> GAMGSMNLLIMGLPGAGKGTQAAKIVEQFHVAHISTGDMFRAAMANQTEMGVLAKSYIDKGELVPDEVTNGIVKERLSQDDI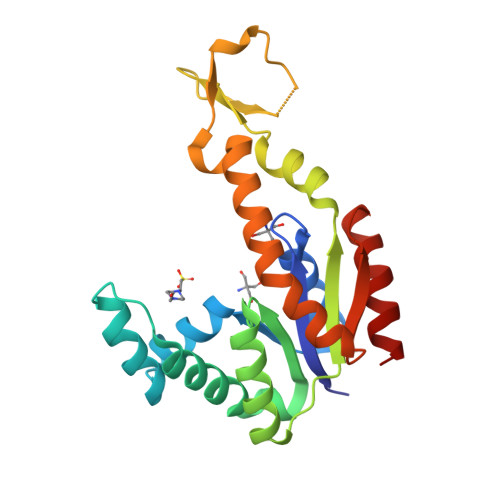KETGFLLDGYPRTIEQAHALDKTLAELGIELEGIINIEVNPDSLLERLSGRIIHRVTGETFHKVFNPPVDYKEEDYYQREDDKPETVKRRLDVNIAQGEPIIAHYRAKGLVHDIEGNQDINDVFSDIEKVLTNLK> MSLSVYEKVNALDKRAIEELFLSEDILMENAAMALERAVLQNASLGAKVIILCGSGDNGGDGYALARRLVGRFRVLVFEMKLTKSPMCQLQKERAKKAGVVIKTYEENALNQNLECDVLIDCVIGSHFKGKLEPFLNFESLSQKARFKIACDIPSGIDSKGRVDKRAFKADLTISMGAIKSCLLSDRAKDYVGELKVGHLGVFNPIYEIPTDTFLLEKSDLKLPLRDKKNAHKGDYGHAHVLLGKHSGAGLLSALSALSFGSGVVSVQALECEITSNNKPLELVFCEN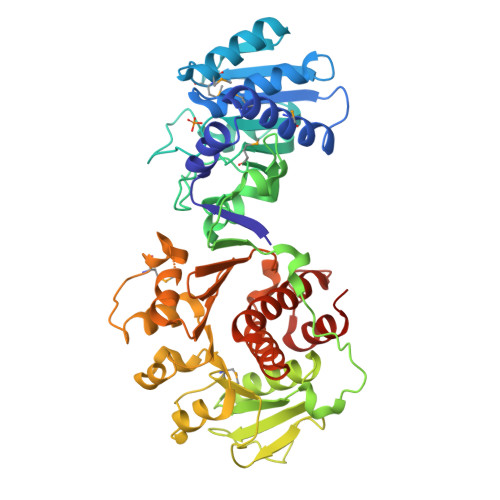FPNLLSAFALGMGLENIPKDFNRWLELAPCVLDAGVFYHKEILQALEKEAVLTPHPKEFLSLLNLVGINISMLELLDNKLEIARDFSQKYPKVVLLLKGANTLIAHQGQVFINILGSVALAKAGSGDVLAGLILSLLSQNYTPLDAAINASLAHALASLEFKNNYALTPLDLIEKIKQLEGHHHHHH> MFKRLMMVALLVIAPLSAATAADQTNPYKLMDEAAQKTFDRLKNEQPQIRANPDYLRTIVDQELLPYVQVKYAGALVLGQYYKSATPAQREAYFAAFREYLKQAYGQALAMYHGQTYQIAPEQPLGDKTIVPIRVTIIDPNGRPPVRLDFQWRKNSQTGNWQAYDMIAEGVSMITTKQNEW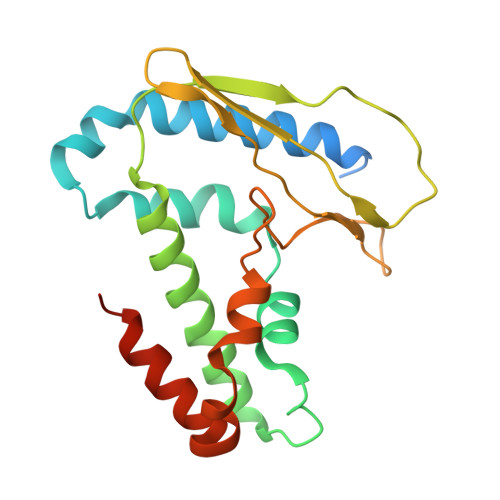GTLLRTKGIDGLTAQLKSISQQKITLEEKK> GDVVEAIEGAVARVADTISSGPTNSQAVPALTAVETGHTSQVVPGDTMQTRHVKNYHSRSESTIENFLSRSACVYMGEYYTTNTDETKRFASWTINARRMVQMRRKLEMFTYVRFDVEVTFVITSKQDQGTQLGQDMPPLTHQIMYIPPGGPIPKSTTDYAWQTSTNPSIFWT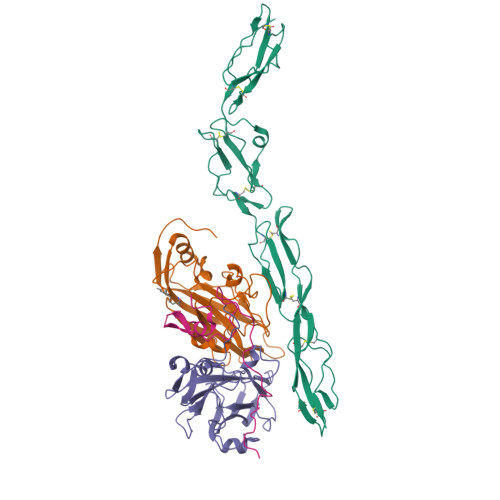EGNAPPRMSIPFVSIGNAYSNFYDGWSHFSQNGVYGYNTLNNMGQLYMRHVNGPSPLPMTSIVRVYFKPKHVKAWVPRPPRLCQYKNASTVNFSSTNITDKRDSITHVPDTVKP;> SPSAEECGYSDRVRSITLGNSTITTQECANVVVAYGRWPEYLSDKEATAEDQPTQPDVATCRFYTLESVTWEKDSPGWWWKFPDALKDMGLFGQNMYYHYLGRAGYTIHVQCNASKFHQGCLLVVCVPEAEMGCSDVGGTVNEHAISEGEIAKKFSATATNGAHTVQSIVTNAGMGVGVGNLTIYPHQWVNLRTNNSATIVMPYINSVPMDNMFRHHNFTLMIIPFVSLDYSSDASTYVPITVTVAPMCAEYNGLRLATSLQ;> GLPVMNTPGSNQFLTSDDFQSPSAMPQFDVTPELDIPGEVKNLMEIAEVDSVVPVNNVVGKLDTMDIFRIPVQSGNHQSTQVFGFQVQPGLDSVFKHTLLGEILNYYAHWSGSVKLTFVFCGSAMATGKFLLAYSPPGANAPKTRKDAMLGTHVIWDVGLQSSCVLCIPWISQTHYRLVHQDEYTSAGNVTCWYQTGIVVPAGTPTLCSIMCFVSACNDFSVRLLKDTPFIEQSALLQ;> MGCVAETGDCGLPPDVPNAQPALEGRTSFPEDTVITYKCEESFVKIPGEKDSVICLKGSQWSDIEEFCNRSCEVPTRLNSASLKQPYITQNYFPVGTVVEYECRPGYRREPSLSPKLTCLQNLKWSTAVEFCKKKSCPNPGEIRNGQIDVPGGILFGATISFSCNTGYKLFGSTSSFCLISGSSVQWSDPLPECREIYCPAPPQIDNGIIQGERDHYGYRQSVTYACNKGFTMIGEHSIYCTVNNDEGEWSGPPPECRGGTKHHHHHH> MVECPVCGSEIEIGEVELHQIVECPVCGAELEVVSLEP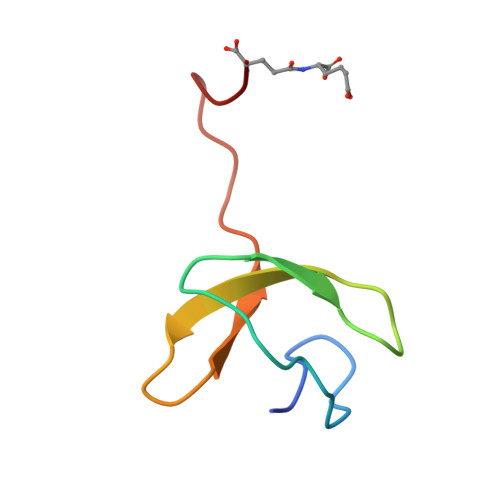LTLEELPEVEEDWGE>[4x]MMSFQKIYSPTQLANAMKLVRQQNGWTQSELAKKIGIKQATISNF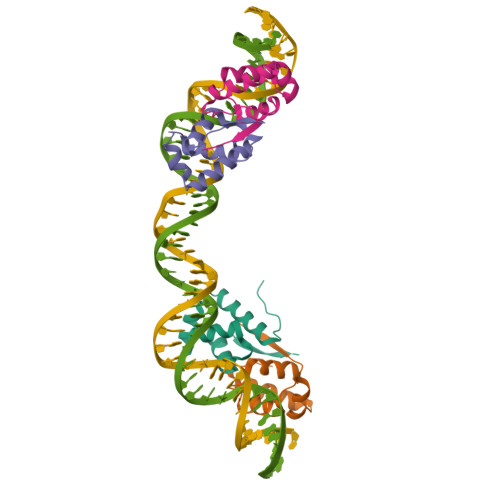ENNPDNTTLTTFFKILQSLELSMTLCD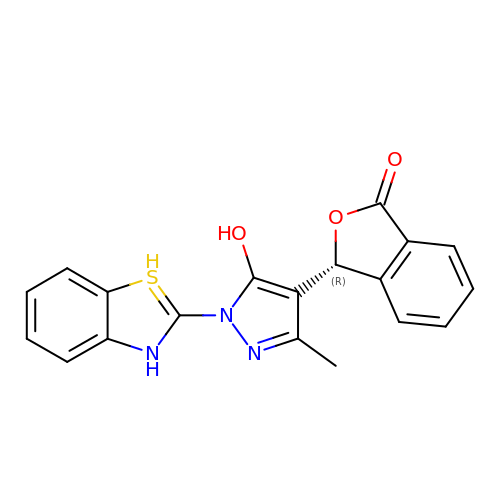(3R)-3-[1-(3H-1lambda~4~,3-benzothiazol-2-yl)-5-hydroxy-3-methyl-1H-pyrazol-4-yl]-2-benzofuran-1(3H)-one | C19 H15 N3 O3 S | LVLUTBWXLVGTPI-MRXNPFEDSA-N> MPIASYAQELKLALHQYPNFPSEGILFEDFLPIFRNPGLFQKLIDAFKLHLEEAFPEVKIDYIVGLESRGFLFGPTLALALGVGFVPVRKAGKLPGECFKATYEKEYGSDLFEIQKNAIPAGSNVIIVDDIIATGGSAAAAGELVEQLEANLLEYNFVMELDFLK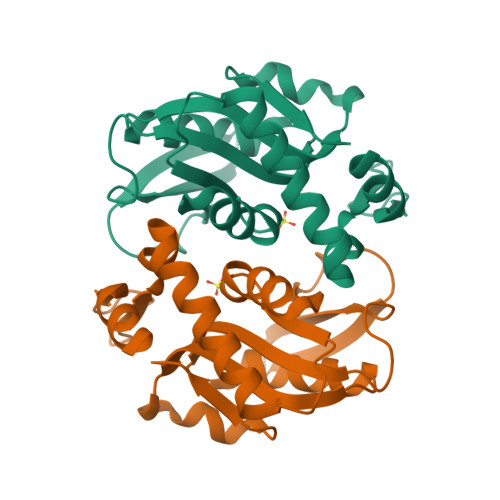GRSKLNAPVFTLLNAQKEALKK>RGSHHHHHHGSEVGTRWAVLVAGSNGYGNYRHQADVCHAYQLLIKGGVKEENIVVFMYDDIAYNAMNPRPGVIINHPQGPDVYAGVPKDYTGEDVTPENLYAVILGDKSKVKGGSGKVINSNPEDRIFIFYSNHGGPGVLGMPNAPFVYAMDFIDVLKKKHASGGYKEMVIYIEACESGSIFEGIMPKDLNIYVTTASNAQENSFGTYCPGMNPPPPEEYVTCLGDLYSVSWMEDSETHNLKRETVQQQYQSVRKRTSNSNSYRFGSHVMQYGDTNITAE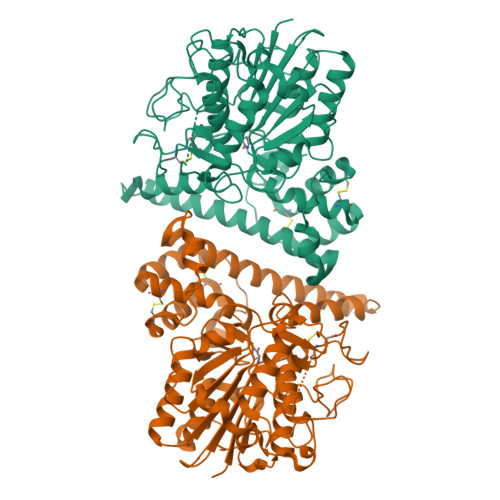KLYLYHGFDPATVNFPPHNGNLEAKMEVVNQRDAELLFMWQMYQRSNHQPEKKTHILEQITETVKHRNHLDGSVELIGVLLYGPGKSSSVLHSVRAPGLPLVDDWTCLKSMVRVFETHCGSLTQYGMKHMRAFGNVCNSGVSKASMEEACKAACGGYDAGLLYPSNTGYSA[2x]> GPLGSAIASEFSSLPSYAAYATAQEAYEQAVANGDSEVVLKKLKKSLNVAKSEFDRDAA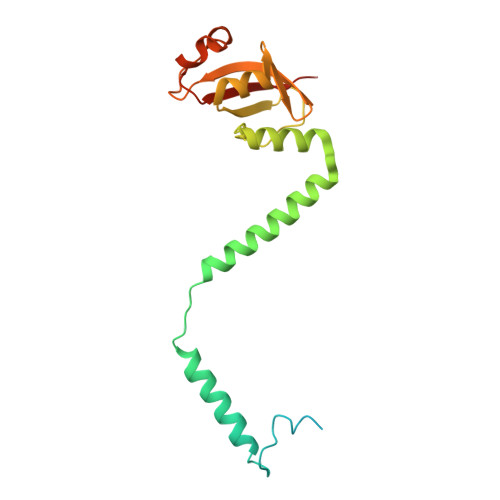MQRKLEKMADQAMTQMYKQARSEDKRAKVTSAMQTMLFTMLRKLDNDALNNIINNARDGCVPLNIIPLTTAAKLMVVVPDYGTYKNTCDGNTFTYASALWEIQQVVDADSKIVQLSEINMDNSPNLAWPLIVTALRANSAVKLQ>MERQVLLSEPEEAAALYRGLSRQPA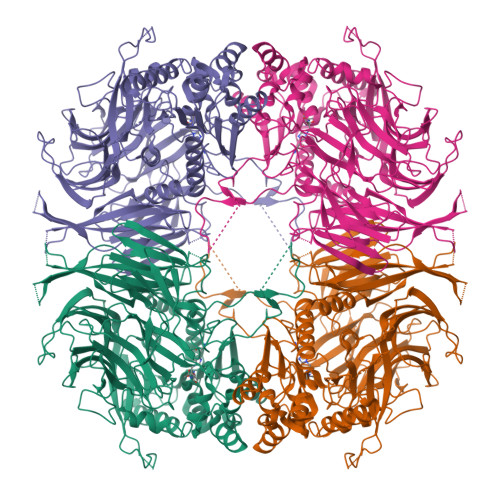LSAACLGPEVTTQYGGRYRTVHTEWTQRDLERMENIRFCRQYLVFHDGDSVVFAGPAGNSVETRGELLSRESPSGTMKAVLRKAGGTGTAEEKQFLEVWEKNRKLKSFNLSALEKHGPVYEDDCFGCLSWSHSETHLLYVADKKRPKAESFFQTKALDVTGSDDEMARTKKPDQAIKGDQFLFYEDWGENMVSKSTPVLCVLDIESGNISVLEGVPESVSPGQAFWAPGDTGVVFVGWWHEPFRLGIRFCTNRRSALYYVDLTGGKCELLSDESVAVTSPRLSPDQCRIVYLRFPSLVPHQQCGQLCLYDWYTRVTSVVVDIVPRQLGEDFSGIYCSLLPLGCWSADSQRVVFDSPQRSRQDLFAVDTQMGSVTSLTAGGSGGSWKLLTIDRDLMVVQFSTPSVPPSLKVGFLPPAGKEQAVSWVSLEEAEPFPDISWSIRVLQPPPQQEHVQYAGLDFEAILLQPSNSPEKTQVPMVVMPHGGPHSSFVTAWMLFPAMLCKMGFAVLLVNYRGSTGFGQDSILSLPGNVGHQDVKDVQFAVEQVLQEEHFDAGRVALMGGSHGGFLSCHLIGQYPETYSACVVRNPVINIASMMGSTDIPDWCMVEAGFSYSSDCLPDLSVWAAMLDKSPIKYAPQVKTPLLLMLGQEDRRVPFKQGMEYYRVLKARNVPVRLLLYPKSTHALSEVEVESDSFMNAVLWLCTHLGS[4x]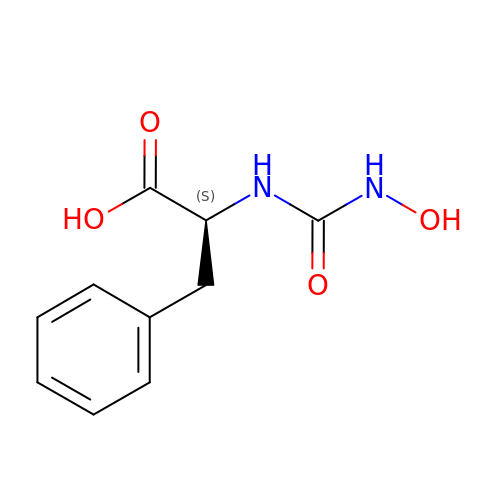L-[(N-HYDROXYAMINO)CARBONYL]PHENYLALANINE | C10 H12 N2 O4 | IOFPEOPOAMOMBE-QMMMGPOBSA-N>[2x]WSLRWRMQKSTTIAAIAGCSGAATFGGLAGGIVGCIAAGILAILQGFEVNWHNGGGGDRSNPV;>[2x]GEATTIWGVGADEA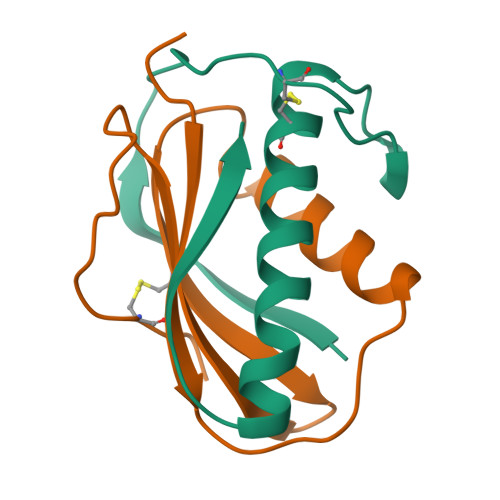IDKGTPSKNDLQNMSADLAKNGFKGHQGVACSTVKDGNKDVYMIKFSLAGGSNDPGGSPCSDD> YRCSGCIAVEKSLNSRNFSKLLHSCPYQCDRHKVIVEAEDRYKSELRKSLIC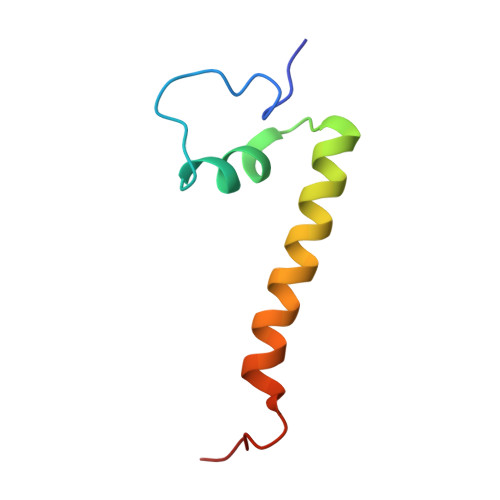NKKILLTP> GSMQVLTKRYPKNCLLTVMDRYSAVVRNMEQVVMIPSLLRDVQLSGPGGSVQDGAPDLYTYFTMLKSICVEVDHGLLPREEWQAKVAGNETSEAENDAAETEEAEEDRISEELDLEAQFHLHFCSLHHILTHLTRKAQ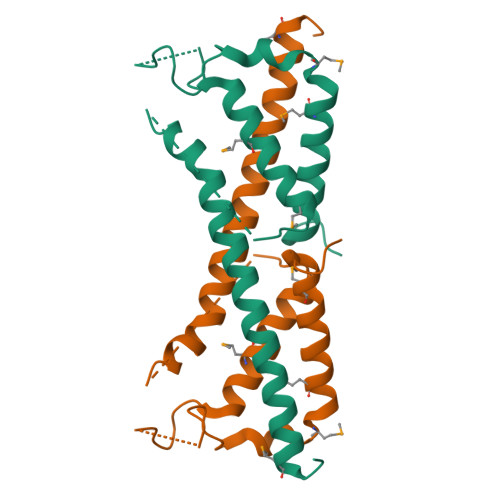EVTRKYQEMTGQVL7-(2-methoxyphenyl)quinazoline-2,4-diamine 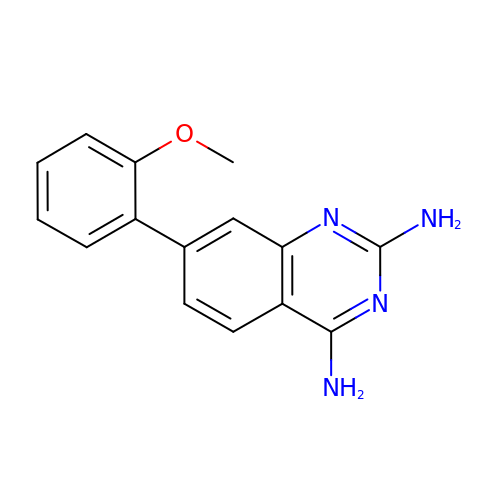| C15 H14 N4 O | GZWYCJUKEDOCPW-UHFFFAOYSA-N>GHMAPLARLAANSARLLQLHKTVPQWHLTDGHLSIKRKFQFSDFNEAWGFMSRVALYADKVDHHPNWYNVYNTVDVELSTHDAAGLTEK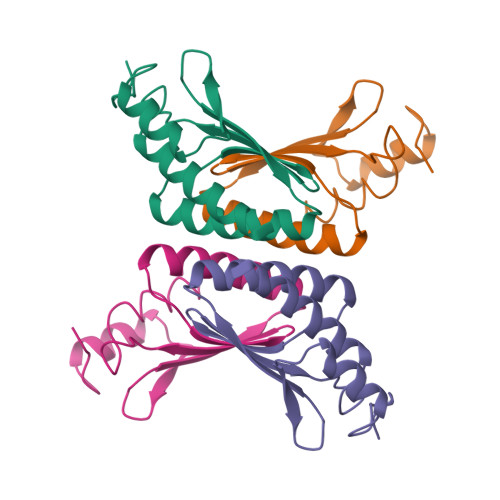DFALAKFMDDAAKNFEK[2x]>[6x]MAWPKVQPEVNIGV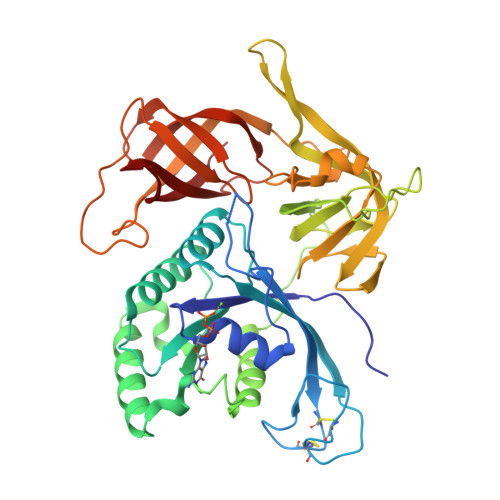VGHVDHGKTTLVQAITGIWTSKHSEELKRGMTIKLGYAETNIGVCESCKKPEAYVTEPSCKSCGSDDEPKFLRRISFIDAPGHEVLMATMLSGAALMDGAILVVAANEPFPQPQTREHFVALGIIGVKNLIIVQNKVDVVSKEEALSQYRQIKQFTKGTWAENVPIIPVSALHKINIDSLIEGIEEYIKTPYRDLSQKPVMLVIRSFDVNKPGTQFNELKGGVIGGSIIQGLFKVDQEIKVLPGLRVEKQGKVSYEPIFTKISSIRFGDEEFKEAKPGGLVAIGTYLDPSLTKADNLLGSIITLADAEVPVLWNIRIKYNLLERVVGAKEMLKVDPIRAKETLMLSVGSSTTLGIVTSVKKDEIEVELRRPVAVWSNNIRTVISRQIAGRWRMIGWGLVEI The gamma-tubulin ring complex (γ-TuRC) is the principal microtubule nucleation template in vertebrates. Microtubules are formed de novo in a process termed nucleation, which is spatially and temporally highly controlled by γ-tubulin complexes, composed of γ-tubulin1 and associated γ-tubulin-complex proteins (GCP). In most eukaryotes, microtubules are templated from a preassembled γ-tubulin ring complex (γ-TuRC) that determines the position and direction of microtubule growth. Here, we used cryo-EM to identify and characterize γ-TuRC assembly intermediates after recombinant expression of the complex, which allowed us to delineate a comprehensive stepwise assembly pathway from a stable 6-spoked core to the mature 14-spoked γ-TuRC, identifying successive stabilization and conformational locking of γ-TuSC units as central principles in the assembly process.

On the GCP2(7)-facing side of the 6-spoke assembly, the expansion phase starts with the recruitment of one γ-TuSC unit, forming spokes 5 and 6 of the fully assembled complex. Notably, the conformation of GCPs in this newly recruited γ-TuSC(5,6) unit differs when compared to the fully assembled complex. In particular, the GRIP2 domains and the associated γ-tubulin copies are displaced from their canonical position. The almost constant ratio between γ-TuSC(13,14)-containing and -lacking intermediates for each assembly step argues for repeated association and dissociation of γ-TuSC(13,14) in an equilibrium reaction.

>MPREIITLQLGQCGNQIGFEFWKQLCAEHGISPEGIVEEFATEGTDRKDVFFYQADDEHYIPRAVLLDLEPRVIHSILNSPYAKLYNPENIYLSEHGGGAGNNWASGFSQGEKIHEDIFDIIDREADGSDSLEGFVLCHSIAGGTGSGLGSYLLERLNDRYPKKLVQTYSVFPNQDEMSDVVVQPYNSLLTLKRLTQNADCVVVLDNTALNRIATDRLHIQNPSFSQINQLVSTIMSASTTTLRYPGYMNNDLIGLIASLIPTPRLHFLMTGYTPLTTDQSVASVRKTTVLDVMRRLLQPKNVMVSTGRDRQTNHCYIAILNIIQGEVDPTQVHKSLQRIRERKLANFIPWGPASIQVALSRKSPYLPSAHRVSGLMMANHTSISSLFERTCRQYDKLRKREAFLEQFRKEDMFKDNFDEMDTSREIVQQLIDEYHAATRPDYISWGTQEQ[10x];>MSEFRIHHDVNELLSLLRVHGGDGAEVYIDLLQKNRTPYVTTTVSAHSAKVKIAEFSRTPEDFLKKYDELKSKNTRNLDPLVYLLSKLTEDKETLQYLQQNAKERAELAAAAVGSSTTSINVPAAASKISMQELEELRKQLGSVATGSTLQQSLELKRKMLRDKQNKKNSGQHLPIFPAWVYERPALIGDFLIGAGISTDTALPIGTLPLASQESAVVEDLLYVLVGVDGRYVSAQPLAGRQSRTFLVDPNLDLSIRELVHRILPVAASYSAVTRFIEEKSSFEYGQVNHALAAAMRTLVKEHLILVSQLEQLHRQGLLSLQKLWFYIQPAMRTMDILASLATSVDKGECLGGSTLSLLHDRSFSYTGDSQAQELCLYLTKAASAPYFEVLEKWIYRGIIHDPYSEFMVEEHELRKERIQEDYNDKYWDQRYTIVQQQIPSFLQKMADKILSTGKYLNVVRECGHDVTCPVAKEIIYTLKERAYVEQIEKAFNYASKVLLDFLMEEKELVAHLRSIKRYFLMDQGDFFVHFMDLAEEELRKPVEDITPPRLEALLELALRMSTANTDPFKDDLKIDLMPHDLITQLLRVLAIETKQEKAMAHADPTELALSGLEAFSFDYIVKWPLSLIINRKALTRYQMLFRHMFYCKHVERQLCSVWISNKTAKQHSLHSAQWFAGAFTLRQRMLNFVQNIQYYMMFEVMEPTWHILEKNLKSASNIDDVLGHHTGFLDTCLKDCMLTNPELLKVFSKLMSVCVMFTNCMQKFTQSMKLDGELGGQTLEHSTVLGLPAGAEERARKELARKHLAEHADTVQLVSGFEATINKFDKNFSAHLLDLLARLSIYSTSDCEHGMASVISRLDFNGFYTERLERLSAERSQKATPQVPVLRGPPAPAPRVAVTAQ[3x];>MATPDQKSPNVLLQNLCCRILGRSEADVAQQFQYAVRVIGSNFAPTVERDEFLVAEKIKKELIRQRREADAALFSELHRKLHSQGVLKNKWSILYLLLSLSEDPRRQPSKVSSYATLFAQALPRDAHSTPYYYARPQTLPLSYQDRSAQSAQSSGSVGSSGISSIGLCALSGPAPAPQSLLPGQSNQAPGVGDCLRQQLGSRLAWTLTANQPSSQATTSKGVPSAVSRNMTRSRREGDTGGTMEITEAALVRDILYVFQGIDGKNIKMNNTENCYKVEGKANLSRSLRDTAVRLSELGWLHNKIRRYTDQRSLDRSFGLVGQSFCAALHQELREYYRLLSVLHSQLQLEDDQGVNLGLESSLTLRRLLVWTYDPKIRLKTLAALVDHCQGRKGGELASAVHAYTKTGDPYMRSLVQHILSLVSHPVLSFLYRWIYDGELEDTYHEFFVASDPTVKTDRLWHDKYTLRKSMIPSFMTMDQSRKVLLIGKSINFLHQVCHDQTPTTKMIAVTKSAESPQDAADLFTDLENAFQGKIDAAYFETSKYLLDVLNKKYSLLDHMQAMRRYLLLGQGDFIRHLMDLLKPELVRPATTLYQHNLTGILETAVRATNAQFDSPEILRRLDVRLLEVSPGDTGWDVFSLDYHVDGPIATVFTRECMSHYLRVFNFLWRAKRMEYILTDIRKGHMCNAKLLRNMPEFSGVLHQCHILASEMVHFIHQMQYYITFEVLECSWDELWNKVQQAQDLDHIIAAHEVFLDTIISRCLLDSDSRALLNQLRAVFDQIIELQNAQDAIYRAALEELQRRLQFEEKKKQREIEGQWGVTAAEEEEENKRIGEFKESIPKMCSQLRILTHFYQGIVQQFLVLLTTSSDESLRFLSFRLDFNEHYKAREPRLRVSLGTRGRRSSHT[6x];>MIHELLLALSGYPGSIFTWNKRSGLQVSQDFPFLHPSETSVLNRLCRLGTDYIRFTEFIEQYTGHVQQQDHHPSQQGQGGLHGIYLRAFCTGLDSVLQPYRQALLDLEQEFLGDPHLSISHVNYFLDQFQLLFPSVMVVVEQIKSQKIHGCQILETVYKHSCGGLPPVRSALEKILAVCHGVMYKQLSAWMLHGLLLDQHEEFFIKQGPSSGNVSAQPEEDEEDLGIGGLTGKQLRELQDLRLIEEENMLAPSLKQFSLRVEILPSYIPVRVAEKILFVGESVQMFENQNVNLTRKGSILKNQEDTFAAELHRLKQQPLFSLVDFEQVVDRIRSTVAEHLWKLMVEESDLLGQLKIIKDFYLLGRGELFQAFIDTAQHMLKTPPTAVTEHDVNVAFQQSAHKVLLDDDNLLPLLHLTIEYHGKEHKADATQAREGPSRETSPREAPASGWAALGLSYKVQWPLHILFTPAVLEKYNVVFKYLLSVRRVQAELQHCWALQMQRKHLKSNQTDAIKWRLRNHMAFLVDNLQYYLQVDVLESQFSQLLHQINSTRDFESIRLAHDHFLSNLLAQSFILLKPVFHCLNEILDLCHSFCSLVSQNLGPLDERGAAQLSILVKGFSRQSSLLFKILSSVRNHQINSDLAQLLLRLDYNKYYTQAGGTLGSFGM[2x];>[2x]MARHGPPWSRLDAQQERDVRELVRGVAGLQDEADPNFQLALNFAWSNFRFHRFLDVNSHKIEKTIEGIYEKFVIHSDLSKAASWKRLTEEFLNAPLPSIKEIKTDAHYSILSLLLCLSDSPSNSSYVETPRNKEVEKKDDFDWGKYLMEDEEMDIGPYMDTPNWSEESEEENDQQPLSREDSGIQVDRTPLEEQDQNRKLDPCISWKDEPDDRSWLEHHVVHQYWTARPSQFPHSLHLHSNLAAVWDQHLYSSDPLYVPDDRVLVTETQVIRETLWLLSGVKKLFIFQLIDGKVTVRNNIIVTHLTHSCLRSVLEQIAAYGQVVFRLQEFIDEVMGHSSESMLPGSGSVPKKSTEAPFRTYQAFMWALYKYFISFKEELAEIEKCIINNDTTITLAIVVDKLAPRLSQLKVLHKVFSTGVAEVPPDTRNVVRASHLLNTLYKAILEYDNVGEASEQTVSLLFSLWVETVRPYLQTVDEWIVHGHLWDGAREFIIQRNKNVPVNHRDFWYATYTLYSVSEKTENEEKMSDNASASSGSDQGPSSRQHTMVSFLKPVLKQIIMAGKSMQLLKNLQCAESTTCQAGARDAERKSLYTLFLESVQSRLRHGEDSTPQVLTEQQATKENLMKMQSIAESHLELDDVHDPLLAINFARMYLEQSDFHEKFAGGDVCVDRSSESVTCQTFELTLRSCLYPHIDKQYLDCCGNLMQTLKKDYRLVEYLQAMRNFFLMEGGDTMYDFYTSIFDKIREKETWQNVSFLNVQLQEAVGQRYPEDSSRLSISFENVDTAKKKLPVHILDGLTLSYKVPWPVDIVISLECQKIYNQVFLLLLQIKWAKYSLDVLLFGELVSTAEKPRLKEGLIHEQDTVAQFGPQKEPVRQQIHRMFLLRVKLMHFVNSLHNYIMTRILHSTGLEFQHQVEEAKDLDQLIKIHYRYLSTIHDRCLLREKVSFVKEAIMKVLNLALMFADGWQAGLGTWRMESIEKMESDFKNCHMFLVTILNKAVCRGSFPHLESLALSLMAGMEQS;> MASITQLFDDLCEALLPAAKTHLGQRSVNRKRAKRSLKKVAYNALFTNLFQDETQQLQPDMSKLPARNKILMLSFDLRVGGLGPKADRLEELVEELEAAPCCPLLEVGSVLDLLVQLAGSGPPQVLPRKRDYFLNNKHVGRNVPYSGYDCDDLSVFEMDVQSLISREECLCHSMIQETLQVMEAAPGTGLPTVGLFSFGDPCGDRFERDTRVSLFGALVHSRTYDMDVRLGLPPVPDNADLSGLAIKVPPSVDQWEDEGFQSASNLTPDSQSEPSVTPDVDLWEAALTYEASKRRCWERVGCPPGHREEPYLTEAGRDAFDKFCRLHQGELQLLAGGVLQAPQPVLVKECELVKDVLNVLIGVVSATFSLCQPAQAFVVKRGVHVSGASPESISSLLSEVAEYGTCYTRLSHFSLQPVLDSLYSKGLVFQAFTSGLRRYLQYYRACVLSTPPTLSLLTIGFLFKKLGRQLRYLAELCGVGAVLPGTCGGGPRAAFPTGVKLLSYLYQEALHNCSNEHYPVLLSLLKTSCEPYTRFIHDWVYSGVFRDAYGEFMIQVNHEYLSFRDKLYWTHGYVLISKEVEDCVPVFLKHIAHDIYVCGKTINLLKLCCPRHYLCWSDVPVPRISVIFSLEELKEIEKDCAVYVGRMERVARHSSVSKEEKELRMEIAKQELIAHAREAASRVLSALSDRQMSERMALDARKREQFQRLKEQFVKDQERRQAARQEELDDDFSYARELRDRERRLKSLEEELERKARQALVDHYSKLSAEAARREQKALWRIQRHRLESARLRFLLEDEKHIQEMLKAVSEAHQPQEPPDVLLSVHPQVTSPGPEHPEGGQGCDSGSAEQHSPAWDGWNRPGLLTPQPLKPLAVGAGGRGLQQAEGARPFSDSLSIGDFLPVGPGAEPSVQTGMVPLLEVALQTINLDLPPSAPGEAPAAASTQPSRPQEYDFSTVLRPAVATSPAPGPLQAAECSLGSSGLQLWEDSCGKMDACGSASRETLLPSHPPRRAALEEGSSQPTERLFGQVSGGGLPTGDYASEIAPTRPRWNTHGHVSDASIRVGENVSDVAPTQPRWNTHGHVSNASISLGESVSDVAPTRPRWNIHGHVSNASIRVGENVSDVAPTRPRWNTHGHVSNASIRVGENVSDVAPTRPRWNTHGHVSDASISLGESVSDMAPARPRWNTHGHVSDASISLGESVSDMAPTRPRWNTHGHVSDTSIRVGENVSDVAPIRSRCNTHGHVSDASISLGEPVSDVVSTRPRWNTHVPIPPPHMVLGALSPEAEPNTPRPQQSPPGHTSQSALSLGAQSTVLDCGPRLPVEVGPSLSSPSSGCGEGSISVGENVSDVAPTQPWWPNTPGDSVSEELGPGRSGDTEDLSPNWPLNSQEDTAAQSSPGRGEEAEASAAEAQGGEQAYLAGLAGQYHLERYPDSYESMSEPPIAHLLRPVLPRAFAFPVDPQVQSAADETAVQLSELLTLPVLMKRSITAPLAAHISLVNKAAVDYFFVELHLEAHYEALRHFLLMEDGEFAQSLSDLLFEKLGAGQTPGELLNPLVLNSVLSKALQCSLHGDTPHASNLSLALKYLPEVFAPNAPDVLSCLELRYKVDWPLNIVITEGCVSKYSGVFSFLLQLKLMMWALKDVCFHLKRTALLSHMAGSVQFRQLQLFKHEMQHFVKVIQGYIANQILHVTWCEFRARLATVGDLEEIQRAHAEYLHKAVFRGLLTEKAAPVMNVIHSIFSLVLKFRSQLISQAWGPPGGPRGAEHPNFALMQQSYNTFKYYSHFLFKVVTKLVNRGYQPHLEDFLLRINFNNYYQDA;>[4x]MASSSGAGAAAAAAAANLNAVRETMDVLLEISRILNTGLDMETLSICVRLCEQGINPEALSSVIKELRKATEALKAAENMTS>[2x]MFLTRRDPPLSSFWTKVQYQRLKELNASGEQLEMGF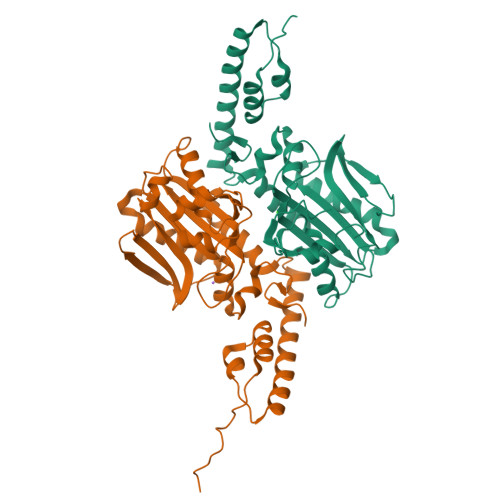SDALSRDRAFQGIEHQLMSQGKRHLEQLRTVKHRPALLELEEKLAKALHQQGFVQVVTPTIITKSALAKMTIGEDHPLFSQVFWLDGKKCLRPMLAPNLYTLWRELERLWDKPIRIFEIGTCYRKESQGAQHLNEFTMLNLTELGTPLEERHQRLEDMARWVLEAAGIREFELVTESSVVYGDTVDVMKGDLELASGAMGPHFLDEKWEIFDPWVGLGFGLERLLMIREGTQHVQSMARSLSYLDGVRLNIN> MSNQGEYPEDNRVGKHEPHDLSLTRRDLIKVSAATAATAVVYPHSTLAASVPAATPAPEIMPLTLKVNGKTEQLEVDTRTTLLDTLRENLHL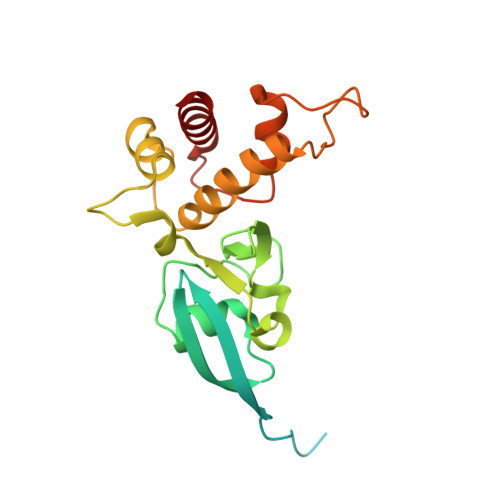IGTKKGCDHGQCGACTVLVNGRRLNACLTLAVMHQGAEITTIEGLGSPDNLHPMQAAFIKHDGFQCGYCTSGQICSSVAVLKEIQDGIPSHVTVDLVSAPETTADEIRERMSGNICRCGAYANILAAIEDAAGEIKS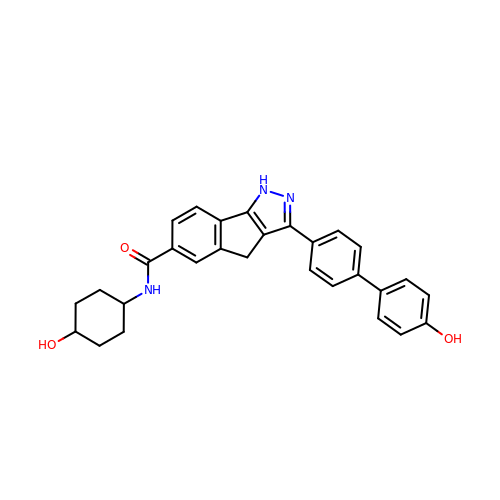3-(4'-HYDROXYBIPHENYL-4-YL)-N-(4-HYDROXYCYCLOHEXYL)-1,4-DIHYDROINDENO[1,2-C]PYRAZOLE-6-CARBOXAMIDE | C29 H27 N3 O3 | VKPCXCHYSBVEMW-HCGLCNNCSA-N>MKGDQKVIEYLNRGLRSELTAVSQYWLHYRMLEDW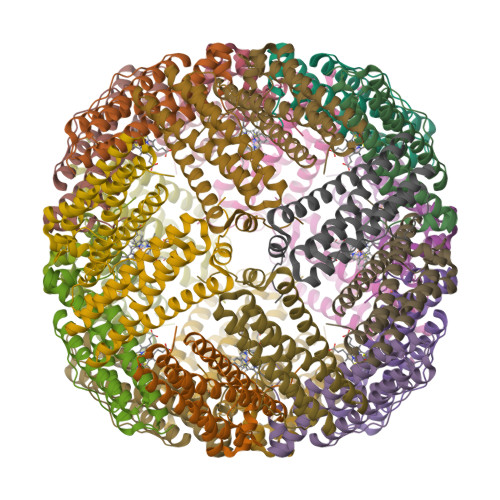GYKDLAKKWRAESIEEMAHADKFVERILFLEGLPNLQTLDPLRIGQTVKEVLESDLAAEREARALYQEGAAYAASVGDFPSKNLFEELMGDEEHHIDFLETQLDLVSKLGLELYAQHHIGKLDD[2x]>GAMARVTMNEFEYLKLLGKGTFGKVILVKEKATGRYYAMKILKKEVIVAKDEVAHTLTENRVLQNSRHPFLTALKYSFQTHDRLCFVMEYANGGELFFHLSRERVFSEDRARFYGAEIVSALDYLHSEKNVVYRDLKLENLMLDKDGHIKITDFGLCKEGIKDGATMKTFCGTPEYLAPEVLEDNDYGRAVDWWGLGVVMYEMMCGRLPFYNQDHEKLFELILMEEIRFPRTLGPEAKSLLSGLLKKDPKQRLGGGSEDAKEIMQHRFFAGIVWQHVYEKKLSPPFKPQVTSETDTRYFDEEFTAQMITITPPDQDD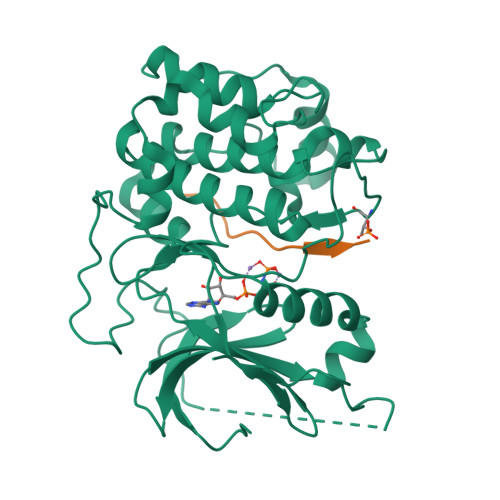SMECVDSERRPHFPQFDYSASSTA[2x];>[2x]GRPRTTSFAE~{N}-[4-(2-azanyl-3-chloranyl-pyridin-4-yl)oxy-3-fluoranyl-phenyl]-5-(4-fluorophenyl)-4-oxidanylidene-1~{H}-pyridine-3-carboxamide 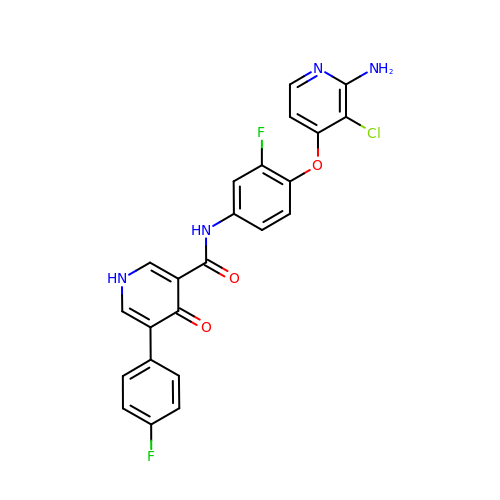| C23 H15 Cl F2 N4 O3 | PDYXPCKITKHFOZ-UHFFFAOYSA-N>MRPERLTVRNFLGLKNVDIEFQSGITVVEGPNGAGKSSLFEAISFALFGNGIRYPNSYDYVNRNAVDGTARLVFQFERGGKRYEIIREINALQRKHNAKLSEILENGKKAAIAAKPTSVKQEVEKILGIEHRTFIRTVFLPQGEIDKLLISPPSEITEIISDVFQSKETLEKLEKLLKEKMKKLENEISSGGAGGAGGSLEKKLKEMSDEYNNLDLLRKYLFDKSNFSRYFTGRVLEAVLKRTKAYLDILTNGRFDIDFDDEKGGFIIKDWGIERPARGLSGGERALISISLAMSLAEVASGRLDAFFIDEGFSSLDTENKEKIASVLKELERLNKVIVFITHDREFSEAFDRKLRITGGVVVNE[4x];>DKL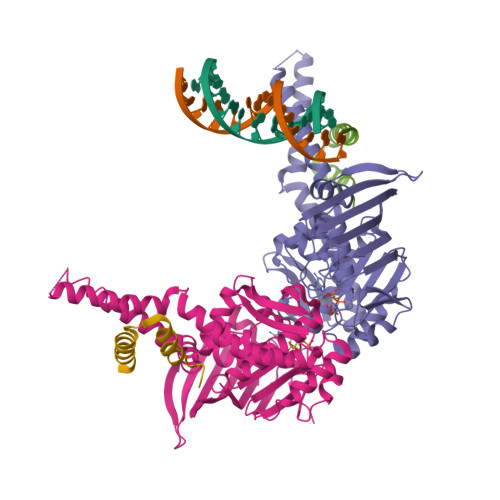DYFELFKEYLKKREENHEKLLKILDELLDEVKKS[4x]~{N}-cyclopropyl-3-oxidanylidene-~{N}-(thiophen-2-ylmethyl)-4~{H}-1,4-benzoxazine-7-carboxamide 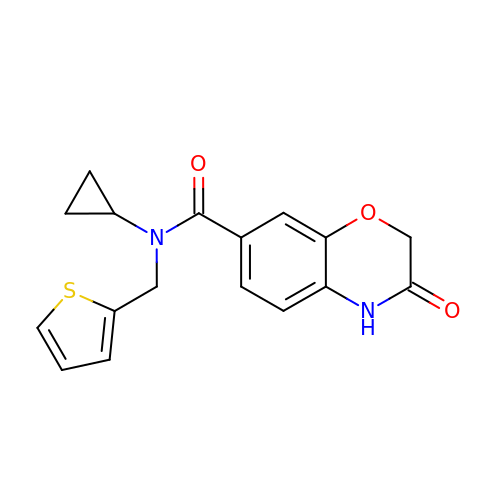| C17 H16 N2 O3 S | XPHOPAPMJBSLFN-UHFFFAOYSA-N>MVNNNRPRRQRAQRVVVTTTQTAPVPQQNVPRNGRRRRNRTRRNRRRVRGMNMAALTRLSQPGLAFLKCAFAPPDFNTDPGKGIPDRFEGKVVSRKDVLNQSISFTAGQDTFILIAPTPGVAYWSASVPAGTFPTSATTFNPVNYPGFTSMFGTTSTSRSNQVSSFRYASMNVGIYPTSNLMQFAGSITVWKCPVKLSTVQFPVATDPATSSLVHTLVGLNGVLAVGPDNFSESFIKGVFSQSACNEPNFQFNDILQGIQTLPPANVSLGSTGQPFTMDSGAEATSGVVGWGNMDTIVIRVSAPEGAVNSAILKAWSCIEYRPNPNAMLYQFGHDSPPLDEVALQEYRTVARSLPVAVIAAQN[3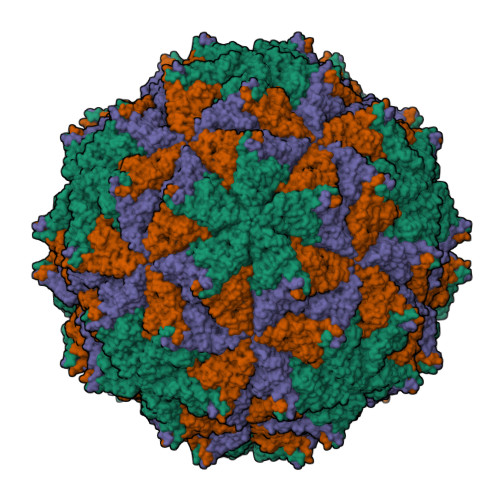x];>ASMWERVKSIIKSSLAAASNIPGPIGVAASGISGLSALFEGFGF[3x]Nucleoporins rich in phenylalanine/glycine (FG) residues form the permeability barrier within the nuclear pore complex and are implicated in several pathological cellular processes, including oncogenic fusion condensates. The self-association of FG-repeat proteins and interactions between FG-repeats play a critical role in these activities by forming hydrogel-like structures. The human nucleoporin Nup98 plays an important role in multiple physiological and pathological processes. The N-terminal 384 residues of human Nup98 (named Nup98FG) comprise two prion-like domains connected by an approximately 50-residue-long linker.

To understand the mechanistic basis of the impact of the F319S mutation on the self-association and aggregation of Nup98FG, we aggregated a 30-residue peptide, which comprises residues 298-327 of Nup98FG, into amyloid fibrils. We subsequently optimized the helical parameters and obtained a map at 2.67 Å resolution. Each layer of the amyloid fibril of Nup98FG(298-327) is formed by five peptides in extended ß-structure-like conformation. Four of the molecules are oriented parallel and one, located at the edge, antiparallel. Side-chains are tightly packed without the presence of internal cavities. One is generated by the 300FSFG303 motif, which forms a four-phenylalanine patch (purple). The second one comprises the 317GLFG320 motif, which contains the mutated F319, and is flanked by two additional hydrophobic residues (methionine and valine). Together they form two zipper-like hydrophobic arrangements in the structure of the Nup98FG(298-327) fibrils (orange). In contrast, the tight zipper-like arrangement of the FG-repeats in the Nup98FG(298-327) fibrils facilitates hydrophobic patch formation with higher stability per residue. This may make it more difficult for nuclear transport receptors to open the FG-repeat meshwork in order to transport cargo across the NPC permeability barrier.

>[25x]TGFSFGNTSTIGQPSTNTMGLFGVTQASQP In Gram-negative bacteria, Fe3+-siderophore complexes are recognised at the bacterial cell surface by highly selective outer-membrane TonB-dependent transporters (TBDTs). These transporters bind the Fe3+-siderophore complex and translocate it into the periplasm. The structures of pyoverdine, pyochelin, citrate and ferrichrome iron complexes bound to their respective transporters FpvA, FptA, FecA and FhuA showed that the ferric-siderophore complexes were bound inside the barrel adjacent to the plug domain, a position thought to be poised for translocation. Pseudomonas aeruginosa, a serious opportunistic pathogen, does not make enterobactin but does possess a TBTD outer-membrane protein PfeA, related to FepA, that binds and translocates Fe3+-enterobactin into the periplasm. PfeA has the same two domains (22-stranded β-barrel and N-terminal plug) common to the TBDTs.

We constructed four mutants R480A, Q482A, G324V and R480A-Q482A (double mutant) to validate the observed recognition site. Each of the mutant proteins was purified as described for the parent protein, and crystal structures of each were obtained. These structures were essentially identical to that of the parent protein, which confirmed that the mutations did not affect the folding of the protein. Neither G324V nor the double mutant were able to form a complex with Fe3+-enterobactin. Unlike the parent protein, the R480A-Q482A double mutant does not coelute with Fe3+-enterobactin. The same titration was carried out with G324V and R480A-Q482A, in both these mutants no binding was detected. A R480A-Q482A double mutant and a more radical G324V mutant have the same structure as the native protein, and did not show any detectable binding to Fe3+-enterobactin (ITC experiments, size-exclusion chromatography and crystallography). Analysis shows that for the double mutant, the lifetime of the Fe3+-enterobactin complex is reduced by four orders of magnitude compared with native (10–3.8 and 100.8 s, respectively) indicating only a transitory interaction. When the double mutant was expressed in bacteria, it was inactive in 55Fe-enterobactin binding and uptake assays. We conclude that the double mutant PfeA is not competent for the uptake of enterobactin in vivo.

> GAMAGQGDGSVIELGEQTVVATAQEETKQAPGVSIITAEDIAKRPPSNDLSQIIRTMPGVNLTGNSSSGQRGNNRQIDIRGMGPENTLILVDGKPVSSRNSVRYGWRGERDSRGDTNWVPADQVERIEVIRGPAAARYGNGAAGGVVNIITKQAGAETHGNLSVYSNFPQHKAEGASERMSFGLNGPLTENLSYRVYGNIAKTDSDDWDINAGHESNRTGKQAGTLPAGREGVRNKDIDGLLSWRLTPEQTLEFEAGFSRQGNIYTGDTQNTNSNNYVKQMLGHETNRMYRETYSVTHRGEWDFGSSLAYLQYEKTRNSRINEGLAGGTEGIFDPNNAGFYTATLRDLTAHGEVNLPLHLGYEQTLTLGSEWTEQKLDDPSSNTQNTEEGGSIPGLAGKNRSSSSSARIFSLFAEDNIELMPGTMLTPGLRWDHHDIVGDNWSPSLNLSHALTERVTLKAGIARAYKAPNLYQLNPDYLLYSAGAGCYGQSTSCYLRGNDGLKAETSVNKELGIEYSHDGLVAGLTYFRNDYKNKIESGLSPVDHASGGKGDYANAAIYQWENVPKAVVEGLEGTLTLPLADGLKWSNNLTYMLQSKNKETGDVLSVTPRYTLNSMLDWQATDDLSLQATVTWYGKQKPKKYDYHGDRVTGSANDQLSPYAIAGLGGTYRLSKNLSLGAGVDNLFDKRLFRAGNAQGVVGIDGAGAATYNEPGRTFYTSLTASF>KGYDSHKIALAQSETEMRNLSHSLAEHATHTFQGADVVLDDIVSFMKWRPHPSPVFNERLRALADNLPQLSDVAILDADGQLTYASVKPVPALDNSDRSYFRYHRANDDHTLLITGPIQSRTSGVWVFVVSRRLETTDGKFFGVVVATIESEYFSTFYKTFDLGPGGSISLLHSDGRLLIQWPSLQTGRDMANMVLFQKALPRSPDGYYLTVSPFDGLTKYLAYRRVSRYPLVVTVART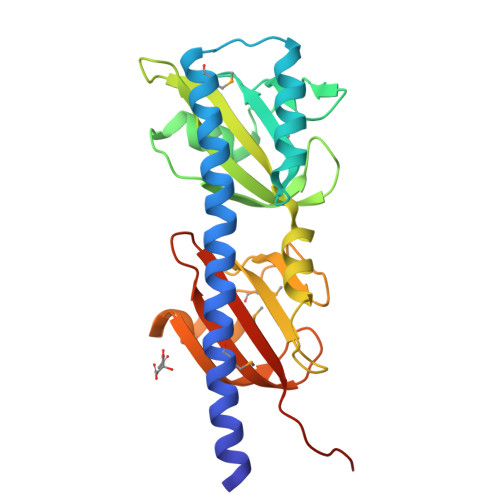EDSVLSGWREAVRSD[2x]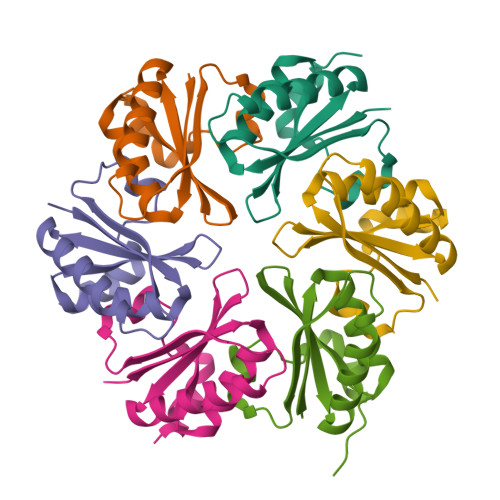>[6x]MAIAVGMIETLGFPAVVEAADAMVKAARVTLVGYEKIGSGRVTVIVRGDVSEVQASVAAGVENVKRVNGGQVLSTHIIARPHENLEYVLPIRYTEAVEQFRELEHHHHHH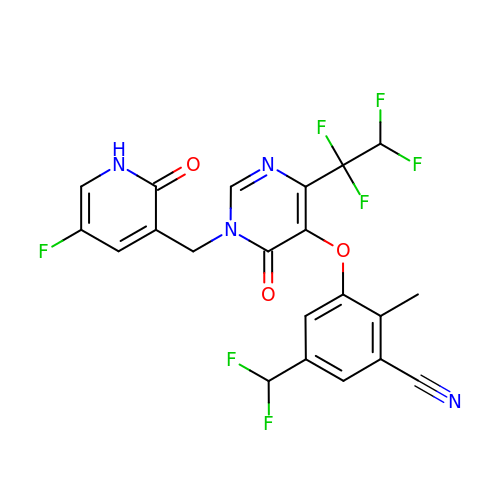5-(difluoromethyl)-3-({1-[(5-fluoro-2-oxo-1,2-dihydropyridin-3-yl)methyl]-6-oxo-4-(1,1,2,2-tetrafluoroethyl)-1,6-dihydropyrimidin-5-yl}oxy)-2-methylbenzonitrile | C21 H13 F7 N4 O3 | VZPBEVWOYXRBLB-UHFFFAOYSA-N>MMIIVGVDAGGTKTKAVAYDCEGNFIGEGSSGPGNYHNVGLTRAIENIKEAVKIAAKGEADVVGMGVAGLDSKFDWENFTPLASLIAPKV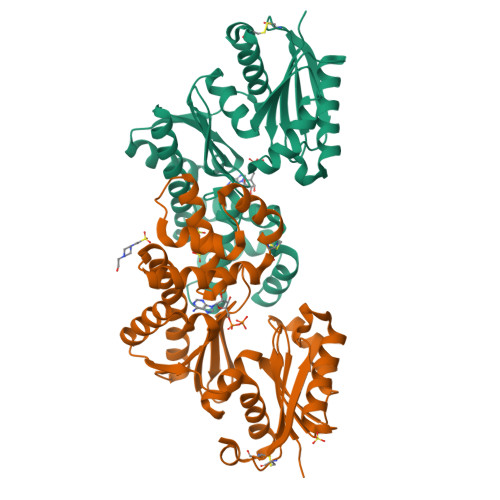IIQHDGVIALFAETLGEPGVVVIAGTGSVVEGYNGKEFLRVGGRGWLLSDDGSAYWVGRKALRKVLKMMDGLENKTILYNKVLKTINVKDLDELVMWSYTSSCQIDLVASIAKAVDEAANEGDTVAMDILKQGAELLASQAVYLARKIGTNKVYLKGGMFRSNIYHKFFTLYLEKEGIISDLGKRSPEIGAVILAYKEVGCDIKKLISD[2x]> GSHMDSTTIQQNKDTLSQIVVFPTG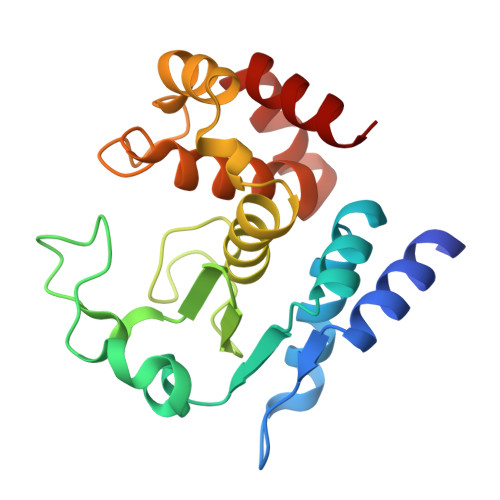NYDKNEANAMVNRLANIDGKYLNALKQNNLKIKLLSGKLTDEKEYAYLKGVVPKGFEGTGKTWDDVPGLGGSTVALRIGFSNKGKGHDAINLELHATAHAIDHIVLNDISKSAQFKQIFAKEGRSLGNVNFLGVYPEEFFAESFAYYYLNQDTNSKLKSACPQTYSFLQNLAK>[2x]MIAAQLLAYYFTELKDDQVKKIDKYLYAMRLSDEILIDILTRFKKEMKNGLSRDYNPTASVKMLPTFVRSIPDGSEKGDFIALDLGGSSFRILRVQVNHEKNQNVSMESEIYDTPENIVHGSGTQLFDHVADCLGDFMEKKKIKDKKLPVGFTFSFPCR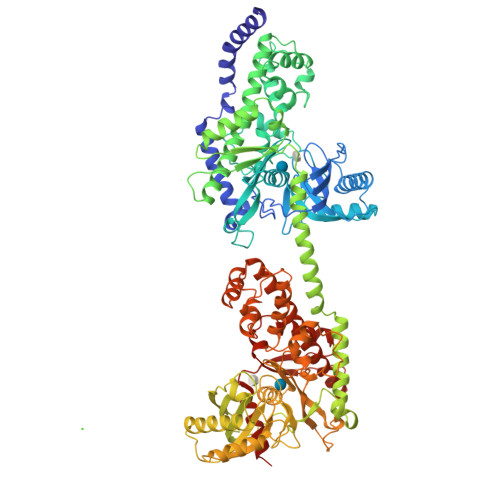QSKIDEAVLITWTKRFKASGVEGADVVKLLNKAIKKRGDYDANIVAVVNDTVGTMMTCGYDDQQCEVGLIIGTGTNACYMEELRHIDLVEGDEGRMCINTEWGAFGDDGSLEDIRTEFDRELDRGSLNPGKQLFEKMVSGMYMGELVRLILVKMAKEGLLFEGRITPELLTRGKFNTSDVSAIEKDKEGIQNAKEILTRLGVEPSDVDCVSVQHICTIVSFRSANLVAATLGAILNRLRDNKGTPRLRTTVGVDGSLYKMHPQYSRRFHKTLRRLVPDSDVRFLLSESGTGKGAAMVTAVAYRLAEQHRQIEETLAHFRLSKQTLMEVKKRLRTEMEMGLRKETNSKATVKMLPSFVRSIPDGTEHGDFLALDLGGTNFRVLLVKIRSGKKRTVEMHNKIYSIPLEIMQGTGDELFDHIVSCISDFLDYMGIKGPRMPLGFTFSFPCHQTNLDCGILISWTKGFKATDCEGHDVASLLRDAVKRREEFDLDVVAVVNDTVGTMMTCAYEEPTCEIGLIVGTGTNACYMEEMKNVEMVEGNQGQMCINMEWGAFGDNGCLDDIRTDFDKVVDEYSLNSGKQRFEKMISGMYLGEIVRNILIDFTKKGFLFRGQISEPLKTRGIFETKFLSQIESDRLALLQVRAILQQLGLNSTCDDSILVKTVCGVVSKRAAQLCGAGMAAVVEKIRENRGLDHLNVTVGVDGTLYKLHPHFSRIMHQTVKELSPKCTVSFLLSEDGSGKGAALITAVGVRLRGDPSIA> MHHHHHHSSGRENLYFQGMTATTRGSPVGGNDNQGQAPDGQSQPPLQQNQTSSPDSSNENSPATPPDEQGQGDAPPQLEDEEPAFPHTDLAKLDDMINRPRWVVPVLPKGELEVLLEAAIDLSKKGLDVKSEACQRFFRDGLTISFTKILTDEAVSGWKFEIHRCIINNTHRLVELCVAKLSQDWFPLLELLAMALNPHCKFHIYNGTRPCESVSSSVQLPEDELFARSPDPRSPKGWLVDLLNKFGTLNGFQILHDRFINGSALNVQIIAALIKPFGQCYEFLTLHTVKKYFLPIIEMVPQFLENLTDEELKKEAKNEAKNDALSMIIKSLKNLASRVPGQEETVKNLEIFRLKMILRLLQISSFNGKMNALNEVNKVISSVSYYTHRHGNPEEEEWLTAERMAEWIQQNNILSIVLRDSLHQPQYVEKLEKILRFVIKEKALTLQDLDNIWAAQAGKHEAIVKNVHDLLAKLAWDFSPEQLDHLFDCFKASWTNASKKQREKLLELIRRLAEDDKDGVMAHKVLNLLWNLAHSDDVPVDIMDLALSAHIKILDYSCSQDRDTQKIQWIDRFIEELRTNDKWVIPALKQIREICSLFGEAPQNLSQTQRSPHVFYRHDLINQLQHNHALVTLVAENLATYMESMRLYARDHEDYDPQTVRLGSRYSHVQEVQERLNFLRFLLKDGQLWLCAPQAKQIWKCLAENAVYLCDREACFKWYSKLMGDEPDLDPDINKDFFESNVLQLDPSLLTENGMKCFERFFKAVNCREGKLVAKRRAYMMDDLELIGLDYLWRVVIQSNDDIASRAIDLLKEIYTNLGPRLQVNQVVIHEDFIQSCFDRLKASYDTLCVLDGDKDSVNCARQEAVRMVRVLTVLREYINECDSDYHEERTILPMSRAFRGKHLSFVVRFPNQGRQVDDLEVWSHTNDTIGSVRRCILNRIKANVAHTKIELFVGGELIDPADDRKLIGQLNLKDKSLITAKLTQISSNMPSSPDSSSDSSTGSPGNHGNHYSDGPNPEVESCLPGVIMSLHPRYISFLWQVADLGSSLNMPPLRDGARVLMKLMPPDSTTIEKLRAICLDHAKLGESSLSPSLDSLFFGPSASQVLYLTEVVYALLMPAGAPLADDSSDFQFHFLKSGGLPLVLSMLTRNNFLPNADMETRRGAYLNALKIAKLLLTAIGYGHVRAVAEACQPGVEGVNPMTQINQVTHDQAVVLQSALQSIPNPSSECMLRNVSVRLAQQISDEASRYMPDICVIRAIQKIIWASGCGSLQLVFSPNEEITKIYEKTNAGNEPDLEDEQVCCEALEVMTLCFALIPTALDALSKEKAWQTFIIDLLLHCHSKTVRQVAQEQFFLMCTRCCMGHRPLLFFITLLFTVLGSTARERAKHSGDYFTLLRHLLNYAYNSNINVPNAEVLLNNEIDWLKRIRDDVKRTGETGIEETILEGHLGVTKELLAFQTSEKKFHIGCEKGGANLIKELIDDFIFPASNVYLQYMRNGELPAEQAIPVCGSPPTINAGFELLVALAVGCVRNLKQIVDSLTEMYYIGTAITTCEALTEWEYLPPVGPRPPKGFVGLKNAGATCYMNSVIQQLYMIPSIRNGILAIEGTGSDVDDDMSGDEKQDNESNVDPRDDVFGYPQQFEDKPALSKTEDRKEYNIGVLRHLQVIFGHLAASRLQYYVPRGFWKQFRLWGEPVNLREQHDALEFFNSLVDSLDEALKALGHPAMLSKVLGGSFADQKICQGCPHRYECEESFTTLNVDIRNHQNLLDSLEQYVKGDLLEGANAYHCEKCNKKVDTVKRLLIKKLPPVLAIQLKRFDYDWERECAIKFNDYFEFPRELDMEPYTVAGVAKLEGDNVNPESQLIQQSEQSESETAGSTKYRLVGVLVHSGQASGGHYYSYIIQRNGGDGERNRWYKFDDGDVTECKMDDDEEMKNQCFGGEYMGEVFDHMMKRMSYRRQKRWWNAYILFYERMDTIDQDDELIRYISELAITTRPHQIIMPSAIERSVRKQNVQFMHNRMQYSMEYFQFMKKLLTCNGVYLNPPPGQDHLLPEAEEITMISIQLAARFLFTTGFHTKKVVRGSASDWYDALCILLRHSKNVRFWFAHNVLFNVSNRFSEYLLECPSAEVRGAFAKLIVFIAHFSLQDGPCPSPFASPGPSSQAYDNLSLSDHLLRAVLNLLRREVSEHGRHLQQYFNLFVMYANLGVAEKTQLLKLSVPATFMLVSLDEGPGPPIKYQYAELGKLYSVVSQLIRCCNVSSRMQSSINGNPPLPNPFGDPNLSQPIMPIQQNVADILFVRTSYVKKIIEDCSNSEETVKLLRFCCWENPQFSSTVLSELLWQVAYSYTYELRPYLDLLLQILLIEDSWQ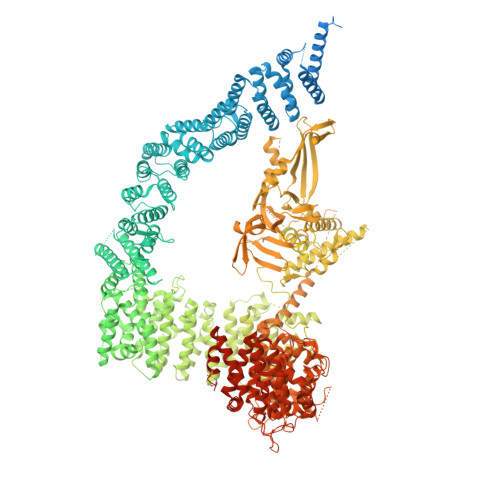THRIHNALKGIPDDRDGLFDTIQRSKNHYQKRAYQCIKCMVALFSNCPVAYQILQGNGDLKRKWTWAVEWLGDELERRPYTGNPQYTYNNWSPPVQSNETSNGYFLERSHSARMTLAKACELCPEEEPDDQDAPDEHESPPPEDAPLYPHSPGSQYQQNNHVHGQPYTGPAAHHMNNPQRTGQRAQENYEGSEEVSPPQTKDQDYKDDDK> ATKAA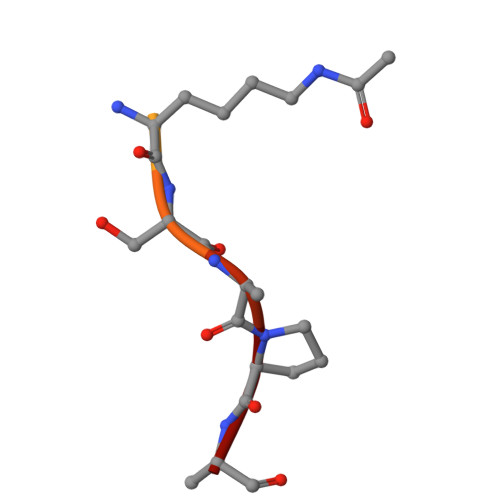RKSAPA Membrane bound histidine kinases (HKs) are ubiquitous sensors of extracellular stimuli in bacteria. Here, we used solid-state NMR in conjunction with crystallography, solution NMR and distance measurements to investigate the transmembrane signaling mechanism of a paradigmatic citrate sensing membrane embedded HK, CitA. In accordance with the naming of the PASc domain, the periplasmic domain is termed PASp here. The PASp and PASc domains are connected to the TM2 helix by two linkers: the PASp/TM2-linker and the TM2/PASc-linker (topology and domain organization shown in Fig. 1A).

We used a bilayer-embedded CitA construct, referred to as the CitApc construct, that contains all essential elements for transmembrane signaling (PASp, TM helices and PASc) and the fully functional R93A mutant. The R93A mutant is used to access the citrate free state, since the wild type cannot be produced without citrate due to very tight binding. Previously, we reported a piston-like motion in the PASp domain along with dynamics changes in the PASc domain of CitA from the thermophilic bacterium Geobacillus thermodenitrificans (GT) upon switching from the free to the bound state by citrate binding. The contraction of the overall β-scaffold of PASp leads to a random coil to α-helix transition in the PASp/TM2-Linker. Based on chemical shift assignment (BMRB ID: 51759 and 51760), we are able to extend this helical characterization to four more amino acids up to I158, which is only one residue away from the predicted membrane embedded region based on cysteine accessibility in the homologous protein DcuS8. This result is in agreement with the conversion of the disordered region downstream of the last β-strand in the PASp core (residues 152-158) in the citrate-free state to a helix (P-helix) extending to the TM2 helix, in the bound state.

>[4x]GSTLKEQIGMRALNVAETVASTSLVREAFRDSNPSVRLQPFAERIRQKTGAEYVVIGNRQGIAYAHPLTERIGKSMIGGDNKEVLKGKSIISEAVGSLGPAIRGKAPIFDENGSVIGIVSVGFLLEDIQRT>MKFKWDEFFVTGDPLILGAQVSIALSTIAIIFVLTYFKKWKWLWSEWITTVDHKKLGIMYIISAVIMLFRGGVDGLMMRAQLALPNNSFLDSNHYNEIFTTHGTIMIIFMAMPFLIGLINVVVPLQIGARDVAFPYLNNLSFWTFFVGAMLFNISFVIGGSPNAGWTSYMPLASNDMSPGPGENYYLLGLQIAGIGTLMTGINFMVTILKMRTKGMTLMRMPMFTWTTLITMVIIVFAFPVLTVALALLSFDRLFGAHFFTLEAGGMPMLWANLFWIWGHPEVYIVILPAFGIFSEIISSFARKQLFGYKAMVGSIIAISVLSFLVWTHHFFTMGNSASVNSFFSITTMAISIPTGVKIFNWLFTMYKGRISFTTPMLWALAFIPNFVIGGVTGVMLAMAAADYQYHNTYFLVSHFHYVLIAGTVFACFAGFIFWYPKMFGHKLNERIGKWFFWIFMIGFNICFFPQYFLGLQGMPRRIYTYGPNDGWTTLNFISTVGAFMMGVGFLILCYNIYYSFRYSTREISGDSWGVGRTLDWATSSAIPPHYNFAVLPEVKSQDAFLHMKEEKTELYPESKFKKIHMPSNSGRPFFMSVAFGLAGFGLVFEWYWMGVVG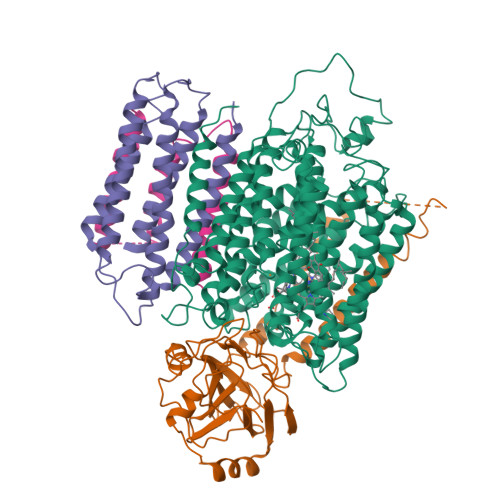LIGVLLCMVLRSFEYDNGYYISVDEIKETERKISEHHHHHH[2x];>[2x]CSNASVLDPKGPVAEQQSDLILLSIGFMLFIVGVVFVLFTIILVKYRDRKGKDNGSYNPEIHGNTFLEVVWTVIPILIVIALSVPTVQTIYSLEKAPEATKDKEPLVVYATSVDWKWVFSYPEQDIETVNYLNIPVDRPILFKISSADSMASLWIPQLGGQKYAMAGMLMDQYLQADKVGTYEGRNANFTGEHFADQEFDVNAVTEKDFNSWVKKTQNEAPKLTKEKYDELMLPENVDELTFSSTHLKYVDHGQDAEYAMEARKRLGYQAVSPHSKTDPFENVKKNEFKKSDDTEE;>MEHAEHGNSNAPMEYQSETGRLNILGFWIFLGAEIVLFSTLFATFFVLKNRTAGGVLPDELFEVNLVMIMTFLLLISSFTCGIAVHEMRRGSLKGVVIWTIITLLLGAGFVGCEINEFVHYVHEGAALSTSAFWSGFFVLLGTHGTHVTIGIFWITGILIQLKKRGLTPQTSSKIFISSLYWHFLDVVWIFIFTGVYLMGLGGL[2x]The pro-survival BCL-2 proteins possess four BH domains (BH1–BH4) and inhibit apoptosis by binding directly to the two sub-classes of pro-apoptotic proteins, BAX/BAK/BOK and BH3-only proteins. BCL-2 proteins are defined by the presence of four regions of sequence homology, the BCL-2 homology domains (BH1–BH4). Based on the C. elegans prototype, nematode BCL-2 proteins inhibit apoptosis by sequestering the apoptosome scaffold protein, CED-4, on mitochondria. We show that the BCL-2-regulated pathway in multiple nematodes is distinct from the classically recognised pathway in C. elegans, with clear evidence for expansion of the multi-BH domain BCL-2-type proteins in some species and notable structural differences in both the BCL-2 and the APAF-1/CED-4 homologues.

Thus, due to the functional importance of this region in C. elegans, we attempted to determine the crystal structure of both BCL-2 proteins of T. suis (designated as T. suis A and T. suis B for convenience), a representative species of clade I. We were only able to obtain crystals for T. suis A and determined its structure to high resolution (1.6 Å), revealing a classic BCL-2-fold consisting of eight α-helices. Helices α3–α4, which line the BH3 binding-groove, are essentially parallel, similar to the apo-BCL-XL structure, though closer together, particularly towards the top of the groove, resulting in a “closed” conformation, as seen in several other BCL-2 structures. The end of α3 is noticeably disordered relative to other apo-BCL-2 structures. The unstructured loop connecting α1–α2, which is significantly shorter in T. suis BCL-2 (and CED-9) compared with BCL-XL and BCL-2, was well-defined and packs primarily against α1, although with some contacts with the beginning of α6. Helix α1 is well-resolved throughout its entire length and its very N-terminal portion is in close proximity to α7, a feature not evident for other BCL-2 protein structures. Helix α8 is also extended relative to that of BCL-XL and is visible through essentially all of the juxta-transmembrane region, which is usually not seen in most BCL-2 structures. Notably, however, the short loop at the α4–α5 junction observed in the CED-9 structure was absent. As this loop is thought to be critical for CED-4 dissociation, this structure indicates that the regulation of apoptosis in T. suis is potentially distinct from C. elegans. Curiously, the loop following helix α4 in CED-9 which is required for release from CED-4 is absent from BCL-2 proteins representing clade I nematodes, as is the case in mammalian BCL-2 proteins which do not directly engage APAF-1. While this observation does not discount the possibility that BCL-2 proteins of clade I nematodes inhibit apoptosome formation in the same manner as occurs in C. elegans, it does suggest that the molecular details of the “release” mechanism are distinct from the free-living nematode.

> GSMSAHNWDNELSGIQNTSVSLAADYVYMRLATEGFVFGIRSSVRAPIRLCDAMFLMCDLFERKFHDRYIAPLKNACLGISAKDMDMRMFFSALDSVFSSGISWSRIVAMYAFAGSVALACARQGRRQTVIAIPEWIMLYMRRAIAPWIHANGGWDSFIKFSQDVLNGNHEEDG>ECQPIFLNVLEAIEPGVVCAGHDNNQPDSFAALLSSLNELGERQLVHVVKWAKALPGFRNLHVDDQMAVIQYSWMGLMVFAMGWRSFTNVNSRMLYFAPDLVFNEYRMHKSRMYSQCVRMRHLSQEFGWLQITPQEFLCMKALLLFSIIPVDGLKNQKFFDELRMNYIKELDRIIACKRKNPTSCSRRFYQLTKLLDSVQPIARELHQFTFDLLIKSHMVSVDFPEMMAEIISVQVPKILSGKVKPIYFHTQ[4x];>MSD[4x];>SLQ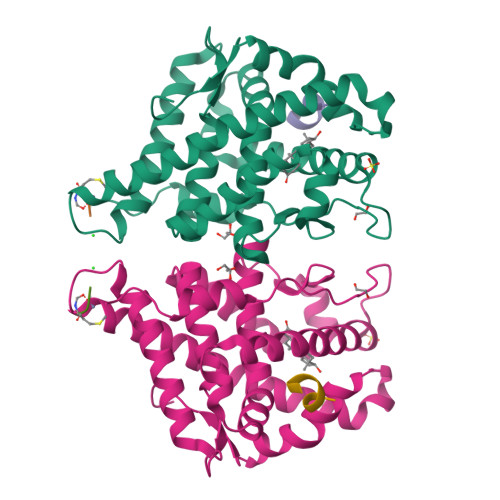FLLDT[4x]> PGGTRIIYD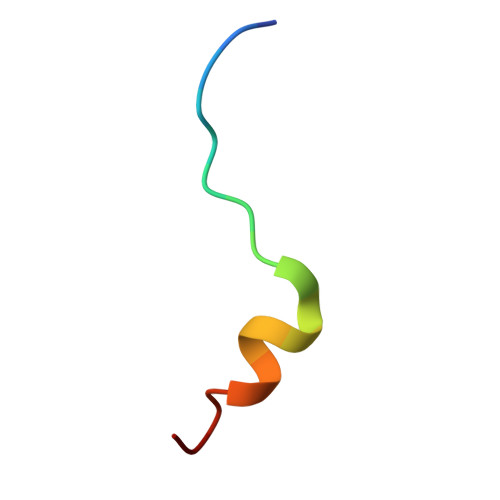RKFLLDRRNS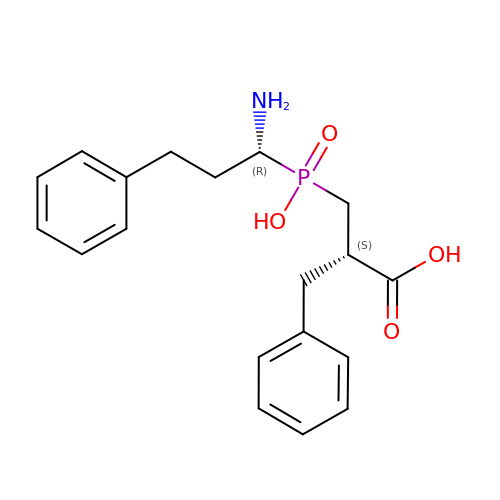(2S)-3-[(S)-[(1R)-1-amino-3-phenylpropyl](hydroxy)phosphoryl]-2-benzylpropanoic acid | C19 H24 N O4 P | QELOIXSGJMIHBZ-QZTJIDSGSA-N> RHLPYFCRGQVVRGFGRGSKQLGIPTANFPEQVVDNLPADISTGIYYGWASVGSGDVHKMVVSIGWNPYYKNTKKSMETHIMHTFKEDFYGEILNVAIVGYLRPEKNFDSLESLISAIQGDIEEAKKRLELPE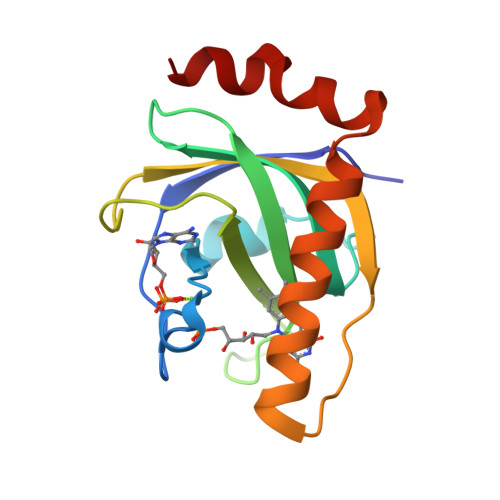YLKIKEDNFFQVSK> AIHEIKQNGNRYKIEKVTDSSLKQALASLRQSAWNVKELDLSGNPLSQISAADLAPFTKLELLNLSSNVLYETLDLESLSTLRTLDLNNNYVQELLVGPSIETLHAANNNISRVSCSRGQGKKNIYLANNKITMLRDLDEGCRSRVQYLDLKLNEIDTVNFAELAASSDTLEHLNLQYNFIYDVKGQVVFAKLKTLDLSSNKLAFMGPEFQSAAGVTWISLRNNKLVLIEKALRFSQNLEHFDLRGNGFHCGTLRDFFSKNQRVQTVAKQTVKKLTGQNEEECTVPTLGHYGAYCCEDLPAPFADRLIALKRKEHALLSGQGSETERLECERENQARQREIDALKEQYRTVIDQVTLRK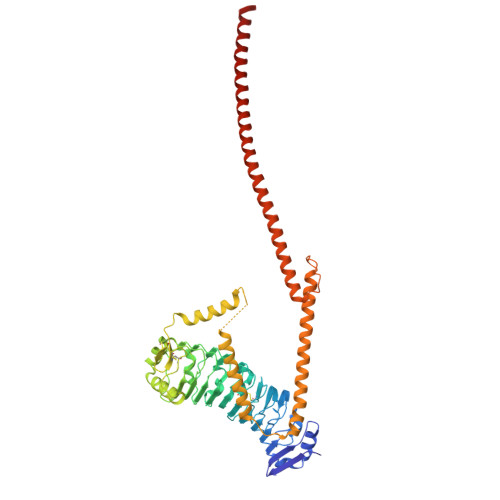QAKITLEQKKKALDEQVSNGRRAHAELDGTLQQAVGQIELQHATEEQSPLQLLRAIVKRYEEMYVEQQSVQNNAIRDWDMYQHKETQLAEENARLKKLNGEADLALASANATLQELVVREQNLASQLG>[2x]HHHHHHSSGLVPRGSHMSTPTPHPQHGVPCGTSTPRPGLLNTPAPGVPFYTPLQSPPSGTALHLSPSTPKLFTPLKIRSL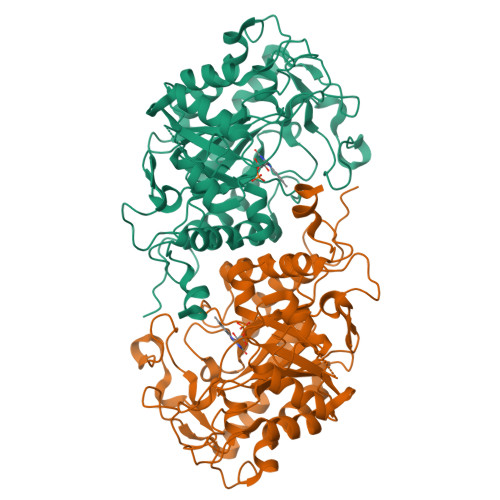TLQNRIMLSPMCQYSASNGHFTPWHMAHLGGIISRGPGLSMVEATSVLPEGRITPEDSGLWLDSQGDKLKEVVQFAHSQGQLIGIQLSHAGRKASMVAPWLDRSAVATEEAGGWPTKVKGPSAIPYDEHHYKPSAMTLEDIQEFKDAWAASLKRALKAGFDVIEIHNAHGYLLHEFVSPVSNKRTDQYGGSFENRIRLTLEIVEITRKIIPESMPLFLRISATDWLDYEGFGEESWTVADSARLAGILADRGVDLMDVSSGANHPRQKITAGLGYQAPFAKEIKRVVGERMLVGTVGMIGSGRQAEGLLSGMGGERGVDEGEEEEGKGTELDLVIVARGFQKNPGLVWEWAEELGVRIMVAHQMRWGFRGKAGGH> HMKELKYDVLIIGGGFAGSSAAYQLSRRGLKILLVDSKPWNRIGDKPCGDAVSKAHFDKLGMPYPKGEELENKINGIKLYSPDMQTVWTVNGEGFELNAPLYNQRVLKEAQDRGVEIWDLTTAMKPIFEDGYVKGAVLFNRRTNEELTVYSKVVVEATGYSRSFRSKLPPELPITEDLDDKDADVAYREVLLTKEDIEDHDYLRIFIDQETSPGGYWWYFPKGKNKVNVGLGIQGGMGYPSIHEYYKKYLDKYAPDVDKSKLLVKGGALVPTRRPLYTMAWNGIIVIGDSGFTVNPVHGGGKGS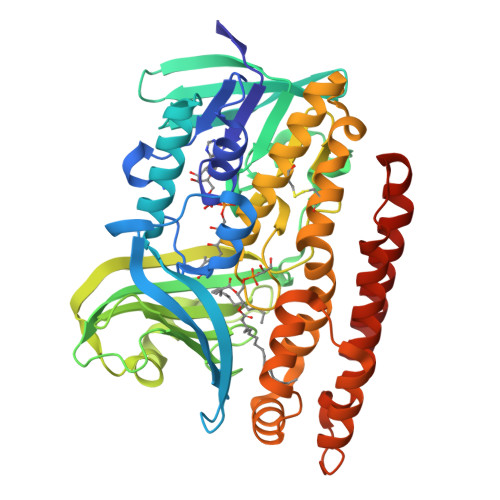AMISGYCAAKAILSAFETGDFSASGLWDMNICYVNEYGAKQASLDIFRRFLQKLSNDDINYGMKKKIIKEEDLLEASEKGDLHLSVADKAMRVISGLGRPSLLFKLKAVAESMKKIKELYLNYPRSPSSLGSWRREVDNVLTEFNKSLS In this work, we exhaustively probe the ability of all 36 immobile HJ sequences to form DNA crystals in two different designed systems. Three separate self-assembling DNA crystal systems are described in this report: the “4 × 5” and “4 × 6” designs (collectively referred to as the 4 × N systems), and a third construct with a “scrambled” sequence variant of the 4 × 6 lattices. Self-assembly was mediated by three constituent oligonucleotides: (S1) containing four sequence repeats of either 5 or 6 bases; (S2) composed of 21 bases containing complementary regions to both (S1); and (S3) which forms the second junction crossover. The HJ serves as the fundamental component at the core of each unit, and the ultimate assembly of the full lattice is facilitated by the complementary 2-base sticky ends that tail each duplex.

To investigate this possibility, we designed “scrambled” sequences with targeted base substitutions, while maintaining GC content, along each “stem”. Contrary to the buffer preference observed with the native P32 crystals, the scrambled systems exhibited an exclusive preference towards low salt buffers, much like the native R3 crystals. Remarkably, only J1 and J2 retained the P32 symmetry, with all others yielding an R3 lattice. It is also noteworthy that J1 and J2 (P32), along with the R3 systems, also shared a preference for low salt conditions, unlike the original P32 crystals. There appeared to be only a marginal difference in the average cell lengths in the R3 scramble crystals (a = b = 113.04 c = 51.10) relative to the native 4 × 6 sequences: the a, b axis trended ~2 Å shorter and c ~1.3 Å longer, whereas in the J1 and J2 cases, the crystals were in good agreement with the original 4 × 6 motif. The average angles of the R3 and P32 crystals were 61.00° (σ = 1.21) and 58.05° (σ = 1.39), respectively. However, in the majority of the crystal structures reported here, the cacodylate anion indeed fits best into the electron density map of our X-ray structures, due to the presence of sodium cacodylate in the crystallization solution.

> GAACGACACTGACGAGGACTC;> TCGTCA;> TCGAGTCC;> GTGTCGT>[235x]MRITFNDVKTSLGITESYDIVNAIRNSQGDNFKSYVPLATANNVAEVGAGILINQTVQNDFITSLVDRIGLVVIRQVSLNNPLKKFKKGQIPLGRTIEEIYTDITKEKQYDAEEAEQKVFEREMPNVKTLFHERNRQGFYHQTIQDDSLKTAFVSWGNFESFVSSIINAIYNSAEVDEYEYMKLLVDNYYSKGLFTTVKIDEPTSSTGALTEFVKKMRATARKLTLPQGSRDWNSMAVRTRSYMEDLHLIIDADLEAELDVDVLAKAFNMNRTDFLGNVTVIDGFASTGLEAVLVDKDWFMVYDNLHKMET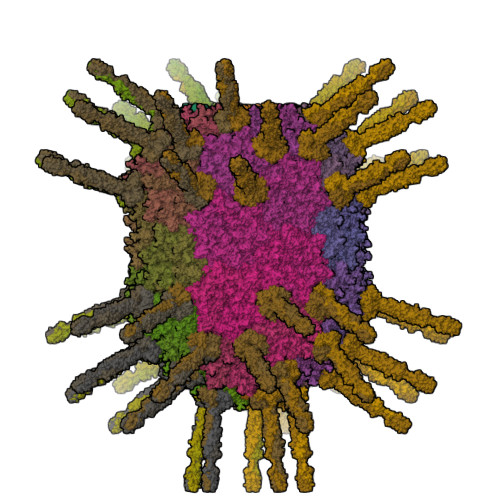VRNPRGLYWNYYYHVWQTLSVSRFANAVAFVSGDVPAVTQVIVSPNIAAVKQGGQQQFTAYVRATNAKDHKVVWSVEGGSTGTAITGDGLLSVSGNEDNQLTVKATVDIGTEDKPKLVVGEAVVSIRPNNASGGAQA;>[165x]MMVSFTARAKSNVMAYRLLAYSQGDDIIEISHAAENTIPDYVAVKDVDKGDLTQVNMYPLAAWQVIAGSDIKVGDNLTTGKDGTAVPTDDPSTVFGYAVEEAQEGQLVTLVISRSKEISIEVEDIKDAGDTGKRLLKINTPSGARNIIIENEDAKALINGETTNTNKKNLQDLLFSDGNVKAFLQATTTDENKTALQQLLVSNADVLGLLSGNPTSDNKINLRTMIGAGVPYSLPAATTTTLGGVKKGAAVTASTATDVATAVKDLNSLITVLKNAGIISL> MKKGSANEDMPVERILEAELAVEPKTETYVEANMGLNPSSPNDPVTNICQAADKQLFTLVEWAKRIPHFSELPLDDQVILLRAGWNELLIASFSHRSIAVKDGILLATGLHVHRNSAHSAGVGAIFDRVLTELVSKMRDMQMDKTELGCLRAIVLF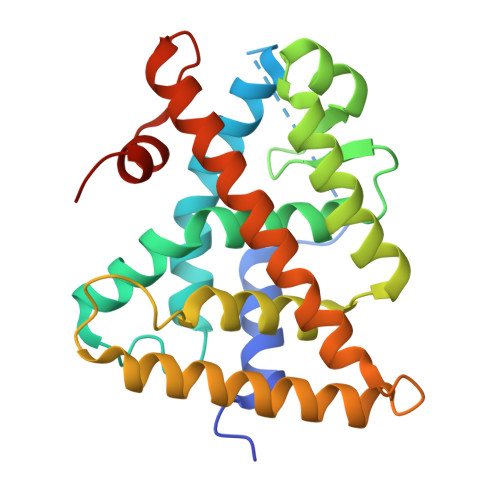NPDSKGLSNPAEVEALREKVYASLEAYCKHKYPEQPGRFAKLLLRLPALRSIGLKCLEHLFFFKLIGDTPIDTFLMEMLEAPHQMTMT>[2x]GGSMNKLYIGNLSENAAPSDLESIFKDAKIPVSGPFLVKTGYAFVDCPDESWALKAIEALSGKIELHGKPIEVEHSVPKRQRIRKLQIRNIPPH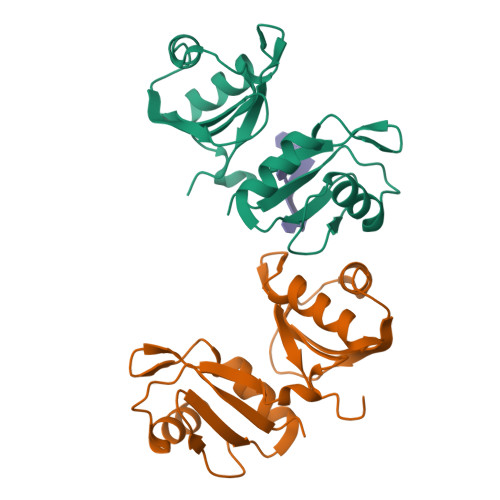LQWEVLDSLLVQYGVVESCEQVNTDSETAVVNVTYSSKDQARQALDKLNGFQLENFTLKVAYIPDEMAAQHHHHHH>MKLDDLNLFRLVVENGSYTSTSKKTMIPVATITRRIQALEDSLNLRLLNRHA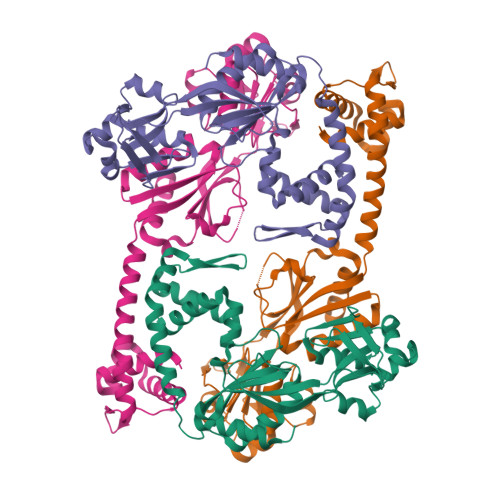RKLTLTEAGERFYKDCSPLLERLASMTEEITDECRGASGRIRISAPSNLTKRMMMPMFNAFMEKYPDIHIELMMSNQADDLDPTEWDVIFRVGPQRDSSLIARKIGEVKDILVASPQYLSSHPQPTHAEELHQHQLLKGYPLLKWQLTNSQGETVVNSDRGRFQASALNVVRSACSEGLGITLMPDVMLREFLEDGSLVQVLSDWSSNPRDIYMLYNHKDHQPEKVRLFIDFVIGYHLQ[2x]>[2x]GSHMKISARNVFKGTVSALKEGAVNAE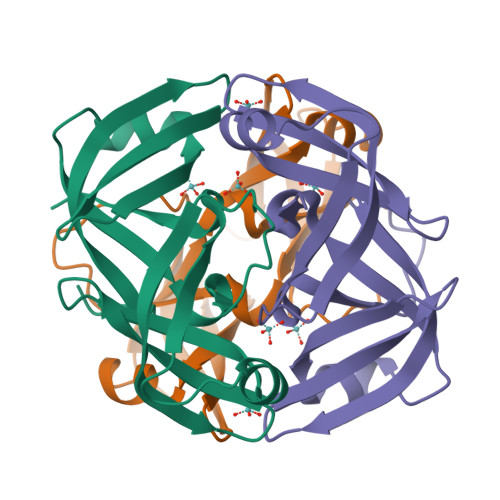VDILLGGGDKLAAVVTLESARSLQLAAGKEVVAVVKAPWVLLMTDSSGYRLSARNILTGTVKTIETGAVNAEVTLALQGGTEITSMVTKEAVAELGLKPGASASAVIKASNVILGVPA>[2x]TSEEPPFDIRALRADIEDMISEKLELGPSLIRLAWHEAASYDCFKKDGSPNSASMRFKPECLYAGNKGLDIPRKALETLKKKYPQISYADLWVLAAYVAIEYMGGP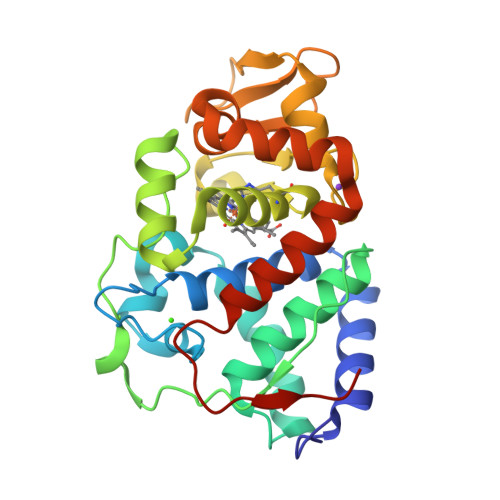TIPFCWGRVDAKDGSVCGPDGRLPDGSKTQSHVREVFRRLGFNDQETVALIGAHTCGECHIEFSGYHGPWTHDKNGFDNSFFTQLLDEDWVLNPKVEQMQLMDRATTKLMMLPSDVCLLLDPSYRKYVELYAKDNDRFNKDFANAFKKLTELGTRNLHKAPASES>[2x]MGSSHHHHHHSSGLVPRGSHMSNQNAPTPPPTEVIQLDWWKNCVLYQIYPRSFKDSDGDGIGDLKGIISELKHFVDAGVDAIWMSPIFESPMVDFGYDISNFYDIHYEYGTMEDFEELLDKAHELGLKVLLDFVPNHASNESEYFIKSEAREPGYENFFIWADPLPNPENPGVRLPPSNWVSQFGGSAWEWSEKRQQYYLHQFAIQQVDFDFRNPAVKQEMFNIMKFWLDKGADGFRLDALPYLIEADPADHEGRYPDDPLSGLTQFESHQLGYTIPLYTKDLIELYDVVYEWREFLDEYNKNHGGDTRVVFSEGYANVSMTMLYYGNEDGAIGAHFPFNFDFITDLSS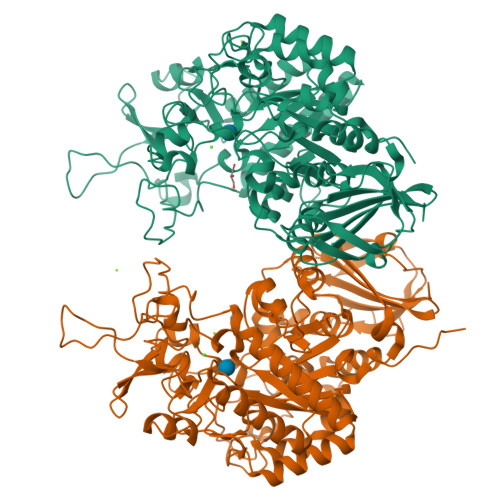KSNARDFVYIILRWLTYMPYGGIPNWVFGNHDNNRMPTRFRHDMVDGLNIINMLLPGVAVTYQGEEIGMRDGYVSWEDTVDIEACNRGDPDTYHLYSRDPARTPYHWDNSTSAGFSTSTNTWLPVAEDYQEINLAKQKETARSHFKNYQALTKLRKQATLSHGEYDIRALSDRTFYLVRSLPTHDTYVLLFNVSERRDTVDLGRVPHLTLPATVYVSSIHSARLAGHEITSSQLSLEAGEALVLKAQPI> GPLGSMLKLSELHDVFQRHPELELKYLNMMKMAITGKESICLPFNFHSHRQHTCLDISPYGNEQVSRIACTSCEDNRILPTASDAMVAFINQTSNIMKNRNFY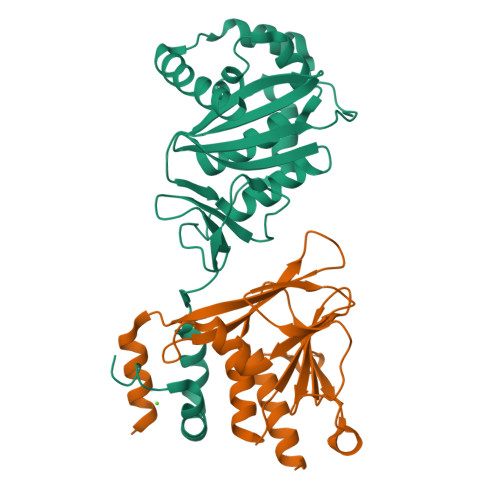YGFCKSSELLKLSTNQPPIFQIYYLLHAANHDIVPFMHAEDGRLHMHVIFENPDVHIPCDCITQMLTAAREDYSVTLNIVRDHVVISVLCHAVSASSVKIDVTILQRKIDEMDIPNDVSESFERYKELIQELCQ;> NKVLHQDLVQATRRILKLGPSELRVTDAGLICKNPNYSVCDAMLKTDTVYCVEYLLSYWESRADHVPCFIFKNTGCAVSLCCFVRAPVALVSPARHVGEFNVLKVNESLIVTLKDIEEIKPSAYGVLTKCVVRKSNSASVFNIELIAFGPENEGEYENLLRELYA> MSYQTKRNVRREARTLMGRFKAGKLAPVMAVPVKGSEGGMLSQSVSFELDPIAGRMATPITAEMCAVFVPVQACDALKNPEADYAGMTEIVREKLLSGNPLFVLEPETDVSKRCGVNPRSNNGLMRVNEIVRLAHNCAVNFLRRRRYVDAVQLTAANHSTTPAILSQTVLDRFNGALDPDPNVNGAVQLSMPDMRLPVASDAEKAVTAPLTVK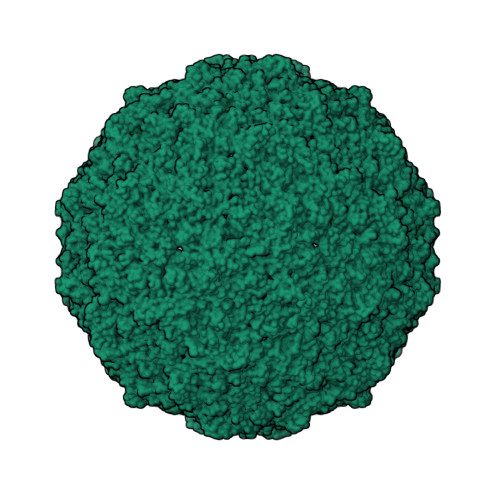RGNENRRLDAGISRLAAAEVAAATDAALYAVFGGREAGNVSLTDFYNAQKMDELTRVMRKICDDNPEYGEEMVLRWAHGLSVDPGRVPFLLAEKSVVLGRQIIGATDTAGVEDGVKRSDMAAQLSFTVPIPTTELGGIIVTFACIKPDETLSSQPHPILADHWRLDNFVADELALDPQPVMARELDYKVAQANETTVVFYTGLNELKKTYVSYGLCRALDPNTVESKNAVWQLEVPLSVTPETVLYPADLPQYPFADQQAEVCTYVVQSTAVMPTPMIFGPSPVEQLAVIETEDLFED>GPLGMLG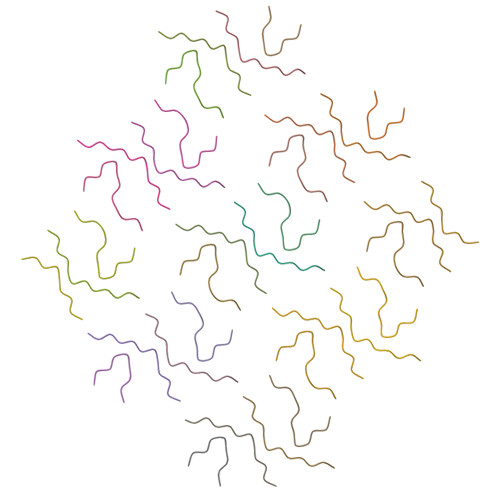GVVIA[34x]>MSVLISGASGYIAKHIVRVLLEQNYKVIGTVRSQDKADKLLKQYNNPNLSYEIVPEIANLDAFDDIFKKHGKEIKYVIHAASPVNFGAKDLEKDLVIPAINGTKNMFEAIKKYAPDTVERVVMTASWASIMTPHRQNDPTLTLDEETWNPVTEENAYENVFTAYCASKTFAEKEAWKFVKENSDAVKFKLTTIHPSFVFGPQNFDEDVTKKLNETCEIINGLLHAPFDTKVEKTHFSQFIDVRDVAKTHVLGFQKDELINQRLLLCNGAFSQQDIVNVFN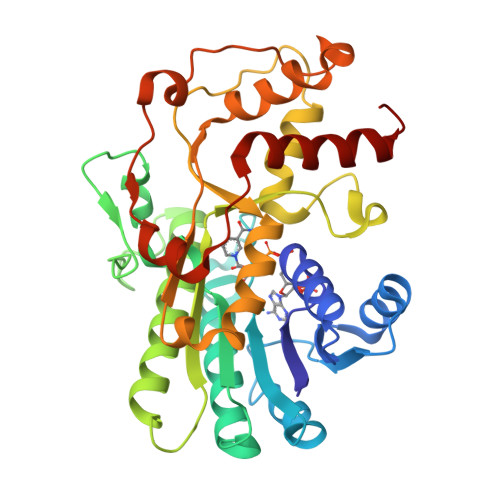EDFPELKGQFPPEDKDTDLNKGVTGCKIDNEKTKKLLAFEFTPFHKTIHDTVYQILHKEGRV[2x]PchD is a stand-alone adenylation enzyme and is part of the initiation module of pyochelin biosynthesis. In the adenylation reaction, salicyl-AMP is formed from salicylate and ATP, releasing pyrophosphate. Next, the thiol of the phosphopantetheinyl (Ppant) prosthetic group of the N-terminal peptidyl carrier protein domain of PchE performs a nucleophilic attack on the carboxyl ester of salicyl-AMP, releasing AMP and transferring the salicyl moiety to the Ppant tether, and priming the first module in the biosynthetic pathway. PchD is comprised of a large N-terminal subdomain (Acore) consisting of residues 1–439 and a smaller C-terminal subdomain (Asub) consisting of residues 441–542 with residue K440 designating the hinge location that allows a range of motion between the two domains.

Using the potent salicyl-AMS inhibitor originally designed by Ferreras et al., the structure of the stand-alone salicylate adenylation domain from Pseudomonas aeruginosa was determined to 2.11 Å. This is the first structure of an adenylation domain bound to the salicyl-AMS inhibitor and serves as an important visual model for making future modifications to continue to develop salicyl-AMS as a therapeutic drug. The co-crystal of PchD and salicyl-AMS diffracted to 2.11 Å resolution and X-ray diffraction data were collected on Stanford Synchrotron Radiation Lightsource beamline 7-1. Analysis of the salicyl-AMS-bound PchD active site revealed that Cys250 is located near to the salicylate ring of salicyl-AMS. The work presented here describes a modification to salicyl-AMS that exploits the presence of an active site cysteine residue near the salicyl ring of the inhibitor. Importantly, both structures were trapped in the catalytically relevant adenylation conformation due to the presence of the inhibitor. PchD overlays very closely with the adenylate-forming conformation of the AB3403 adenylation domain with an rmsd of 2.03 Å over 438 Cα. The Asub of PchD is comprised of a central three stranded β-sheets surrounded by three helices. Regardless of the ligand bound, the two structures are in identical conformation with an rmsd of 0.15 Å over 523 Cα.

> MTSSPVTPSAVDDAPDWPAAFVRRYLDAGHWQDQSFAEALATSAARHPRRIALCDDDQRLSYADLLQRCRRLAAGLRQAGLAHGDTVVLHLPNGIAFVETCFALFQLGVRPVLALPAHRQHEISGFCRFAEAKAYIGAERIDGFDPRPMARELLASGACRMALIHGEAEAPLQALAPLYQADALEDCAARAEDIACFQLSGGTTGTPKLIPRRHREYLYNVRASAEVCGFDEHTVYLTGLPMAHNFTLCCPGVIGTLLASGRVVVSQRADPEHCFALIARERVTHTALVPPLAMLWLDAQESRRADLSSLRLLQVGGSRLGSSAAQRVEPVLGCQLQQVLGMAEGLICYTRLDDPPERVLHTQGRPLSPDDEVRVVDAEGREVGPGEVGELTVRGPYTIRGYYRLPEHNAKAFSADGFYRTGDRVSRDKDGYLVVEGRDKDQINRGGEKIAAEEVENLLIAHPQVHDATVVAMPDSLLGERTCAFVIPRQPAPSALKLKQYLHACGLAAFKVPDRIELVPAFPQTGIGKISKKDLRERLRRELEARA> MRGKILIFLHAHLPYVHHPEYDHFLEERWLFEAITETYIPLLMMFDEIEDFRLTMSITPPLMEMLSSRDLQEKYERHMEKLIELANKEVERTKKEHPLKHKMAKFYREHFEKILNVFRSYDGNILEGFKKYQETGKLEIVTCNATHAFLPLYQMYPEVVNAQITVGVKNYEKHMKKHPRGIWLAECGYYQGLDLYLAQNNVEYFFVDSHAFWFADEQPRYGVYRPIMTPSGVFAFARDPESSEQVWSAAVGYPGDPRYREFYRDIGFDREMEYIKDYIDPSGVRINTGIKYHRITSKSLDASQKEYYDIDLAMEAVEEHARDFLHKKESQA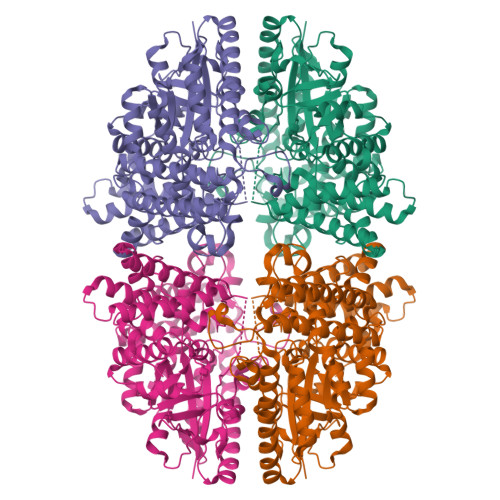RRLMDIMGVEPVIVAPFDAELFGHWWFEGVFFLKRFFELVNESKDLKLVTASEVIDTLEEVQIATPADSSWGAGGYYETWLNGTNDWIYRHLHEMIERMIDLSKKYYNSSDPLVERVLNQMLRELFLAQSSDWAFIMTTRTSVQYAENRTKLHIKRFLNLYDQLVSGRIDEEMLRYYEWTDAIFPEINFRVMARDVI> 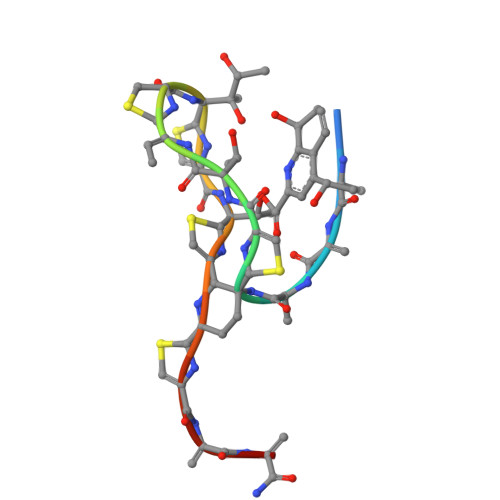XIASASCTTCICTCSCSSX> KSCCKSTLGRNCYNLCRARGAQKLCANVCRCKLTSGLSC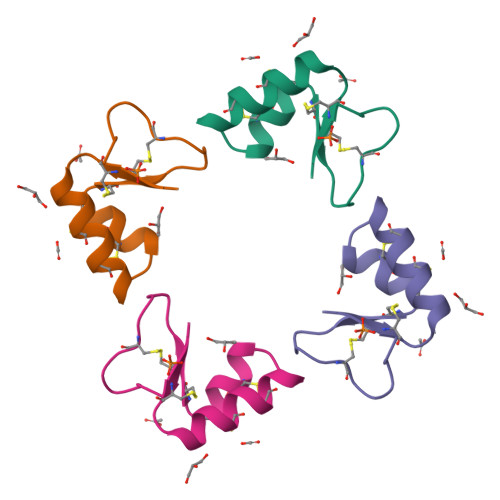PKDFPK> MHHHHHHLVPRGSVSKRDKRISLDDAVGELRSGMTIGIGGWGSRRKPMALVRALLRSDVTDLTVVTYGGPDLGLLCSAGKVTKAYYGFVSLDSAPFYDPWFAKARTAGEIAVREMDAGMVKCGLEAAAARLPFLPIRAGLGSDVRRFWGDELRTVTSPYPDASGKSETLIAMPALNLDAALVHLNLGDKHGNAAYTGVDPYFDDLYCAAAEKRFVSVERVVETEELVKTV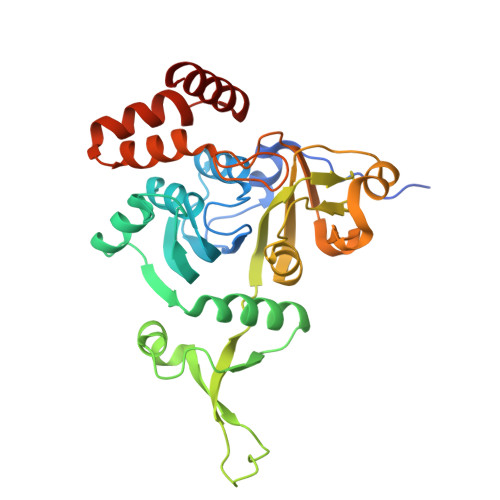PLQNLILNRMMVDGVVEAPNGAHFTLAGDSYGRDEKFQRHYAESAKTPQAWQQFVATYLSGSEDDYQAAVKKFAEEQA>MHHH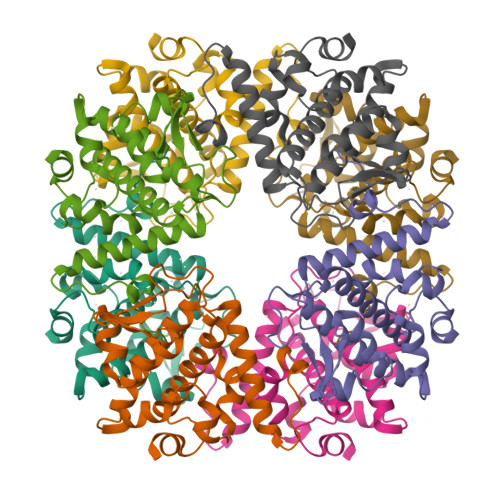HHHSSGRENLYFQGMPGEEEERAFLVAREELASALRRDSGQAFSLEQLRPLLASSLPLAARYLQLDAARLVRCNAHGEPRNYLNTLSTALNILEKYGRNLLSPQRPRYWRGVKFNNPVFRSTVDAVQGGRDVLRLYGYTEEQPDGLSFPEGQEEPDEHQVATVTLEVLLLRTELSLLLQNTHPRQQALEQLLED[2x]>[2x]GPQPMSSQIPSLKDVFLQDFKIGVALPVRVFSNSMDVELITKHFNSMTAENEMKPESILRRDASGKIYYDFTVADRYIEFAQKHGMVVRGHTLVWHSQTPEWFFKDEKGNLLSREAMIERMREYIHTVVGRYRGKVYAWDVVNEAVDENQPDGLRRS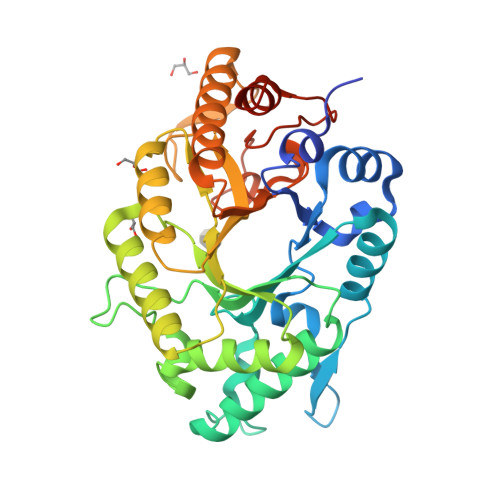LWYQVIGPDYIELAFKFAHEADPDALLFYNDYNEFFPKKRDIIFKLVKEMREKGVPIHGIGMQQHLTLADNVGWIDIAIQKFKTISGIQIHITELDVSVYKSRSPSIIYQTPPLEVLKEQAEFYRKLFEIYRKHTDVITNVTFWGLKDDYSWLRFFFGRRNDWPLLFDENYQPKPAFWSVIESVSKVDLQPSLIS> SNAMYGISVFLGEEITNDTIIYIKKMKALGFDGIFTSLHIPEDDTSLYRQRLTDLGAIAKAEKMKIMVDISGEALKRAGFSFDELEPLIELGVTGLRMD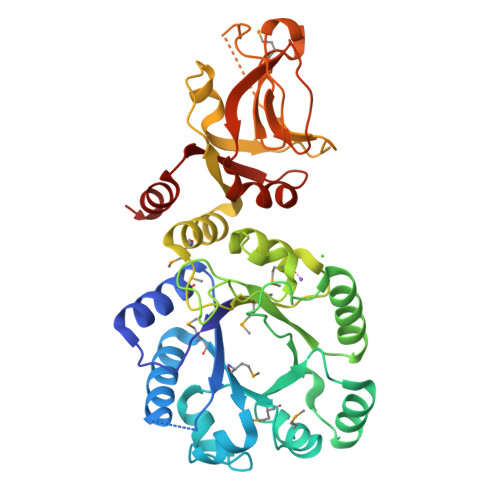YGITIEQMAHASHKIDIGLNASTITLEEVAELKAHQADFSRLEAWHNYYPRPETGIGTTFFNEKNRWLKELGLQVFTFVPGDGQTRGPIFAGLPTLEKHRGQNPFAAAVGLMADPYVDAVYIGDPTISERTMAQFGYYHQTNQFLLEVAPSESRYLKRILGTHTNRLDAARDVLRSELSRTSEMFRKDEIATIESEQTEARPVGTVTIDNEKYGRYMGEIQVTLVDLPKDEKVNTITRIIDKDQTILPLIKAGNQFTLVTEGTIENEFRKLNN> MGSDKIHHHHHHENLYFQGMELLIRTEQLLLQNEKNWELYLSNREEEKPFDFYKDMKPFVD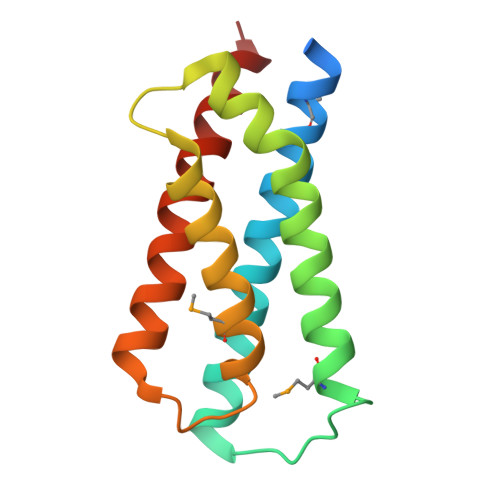EAKRCADDFLELAIPWVNTERPPYLGELQLRQACDNVQMTAVSAFNGRSFYKHFLDHYQSTKYTLTRVRDFLKRKEESM3-amino-N-(5-phenyl-1,3,4-thiadiazol-2-yl)-6,7,8,9-tetrahydro-5H-cyclohepta[b]thieno[3,2-e]pyridine-2-carboxamide | C21 H19 N5 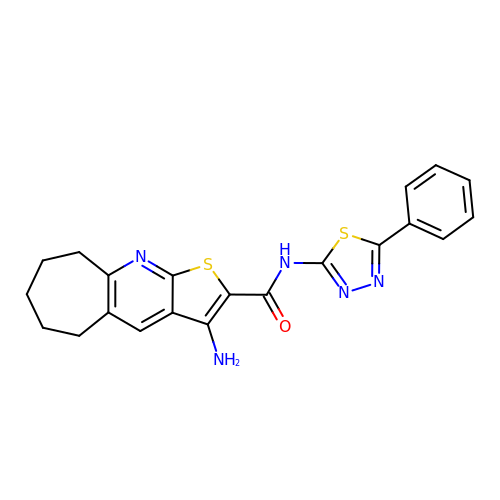O S2 | FGRXYHXHXBKKAK-UHFFFAOYSA-N>MFKRFSKKKEAPEDPKNLINIDKPIKELPASIAIPKEKPLTGEQQKMYDEVLKHFSNPDLKVYTSEKNKSEDDLKPLEEEEKAWLTRECFLRYLRATKWVLKDCIDRITMTLAWRREFGISHLGEEHGDKITADLVAVENESGKQVILGYENDARPILYLKPGRQNTKTSHRQVQHLVFMLERVIDFMPAGQDSLALLIDFKDYPDVPKVPGNSKIPPIGVGKEVLHILQTHYPERLGKALLTNIPWLAWTFLKLIHPFIDPLTREKLVFDEPFVKYVPKNELDSLYGGDLKFKYNHDVYWPALVETAREKRDHYFKRFQSFGGIVGLSEVDLRGTHEKLLYPVKSESSTVL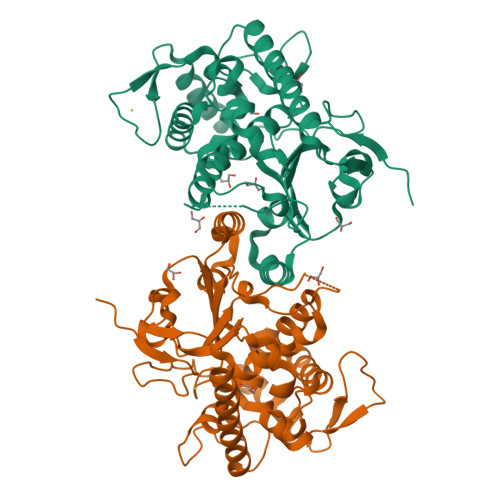EHHHHHHH[2x]> MEEKKRLHLIIADAELETVPPEILDHPAIVNYAKRRKKRPEKIILDSTYHHAALRQLEDGERRGRPDIVHICLLNALDSILNKEDRLRVYVHTRNDYVIYIKPETRLPRNYNRFIGLMENLFEKGAVPEDLELLRMEKKT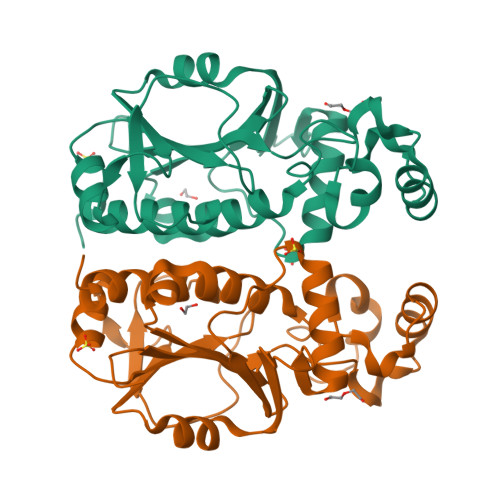LNELIEEINPDVVFIMHEEGELMIPKNFGKLLDKFKKPTVIVGGFPHGDFKSKVDGVKISLYREPLMAWTIVNEVIVSYEWEVIKKFKS>[2x]SNAMKQLTILGSTGSIGNSTLSVVRANPELFKVTALVAGRNVREMAQQCLEFSPRYAAMSDEH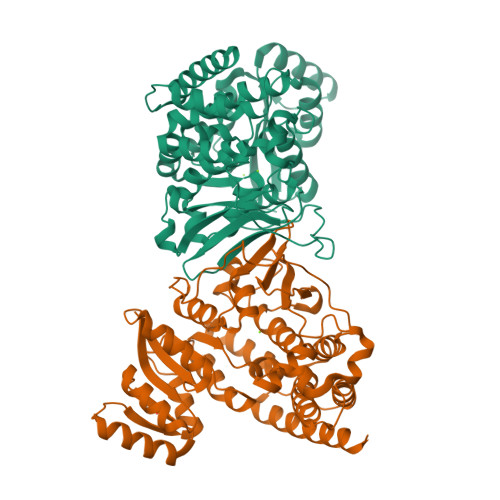SAKSLRLLLAEQGSDTEVYSGETAACELAALDDVDQVMAAIVGIAGLPSTLAAIRAGKQVLLANKESLITCGKLFMDEVKRSRAQLLPIDSEHNAIFQSLPERIQRQLGYSSLNENGVSRIILTGSGGPFRETPLSQFSDVTPDQACAHPNWSMGRKISVDSATMMNKGLEYIEARWLFNASAEQIEVVLHPQSVIHSMVRYHDGSILAQMGTPDMRTPIAHAMAYPMRVSSGVAPLDFCKVGALTFTTPDYQRYPCLKLAIDACNAGQAATTALNAANEISVMAFLDSKIRFTDIEVINRTVVEGLLLSEPTSVEEVLVIDRKARDVAAQVIAKLNN> IVGGYTCEENSLPYQVSLNSGSHFCGGSLISEQWVVSAAHCYKTRIQVRLGEHNIKVLEGNEQFINAAKIIRHPKYNRDTLDNDIMLIKLSSPAVINARVSTISLPTAPPAAGTECLISGWGNTLSFGADYPDELKCLDAPVLTQAECKASYPGKITNSMFCVGFLEGGKDSCQRDAGGPVVCNGQLQGVVSWGHGCAWKNRPGVYTKVYNYVDWIK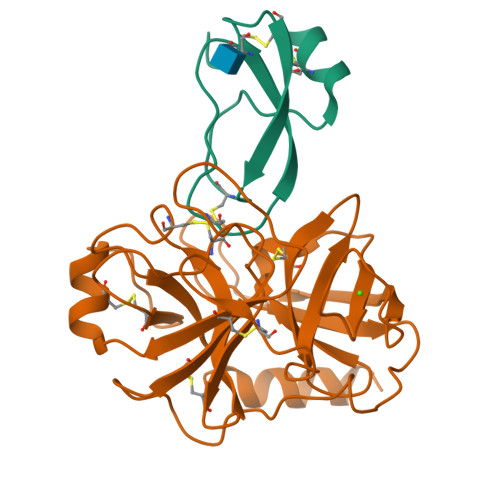DTIAANS;> IHDFCLVSKVVGRCRASMPRWWYNVTDGSCQLFVYGGCDGNSNNYLTKEECLKKC> SSVVVDTNGQPVSNGADAYYLVPVSHGHAGLALAKIGNEAEPRAVVLDPHHRPGLPVRFESPLRINIIKESY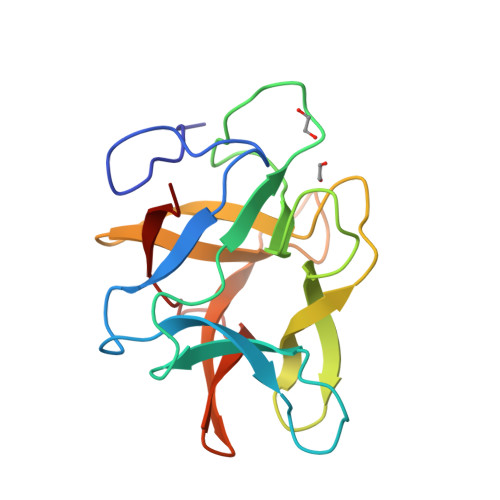FLNIKFGPSSSDSGVWDVIQQDPIGLAVKVTDTKSLLGPFKVEKEGEGYKIVYYPERGQTGLDIGLVHRNDKYYLAVKDGEPCVFKIRKAT>[2x]MFLLQAPLQRRILEIG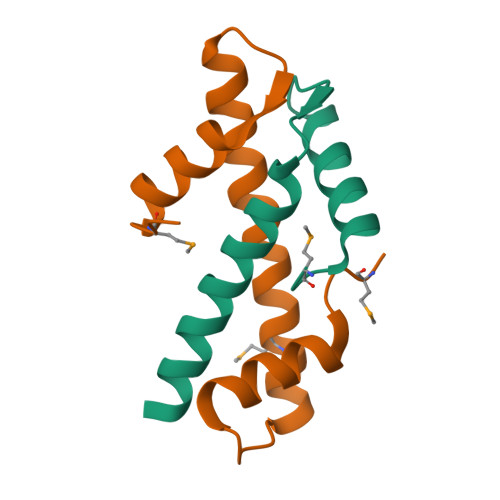KKHGITELHPDVVSYVSHATQQRLQNLVEKISETAQQKNFSYKDDDRYEQASDVRAQLK;>GSHMVLTKKKLQDLVREVDPNEQLDEDVEEMLLQIADDFIESVVTAACQLARHRKSSTLEVKDVQLHLERQWNMWI[2x]>[4x]MAGTST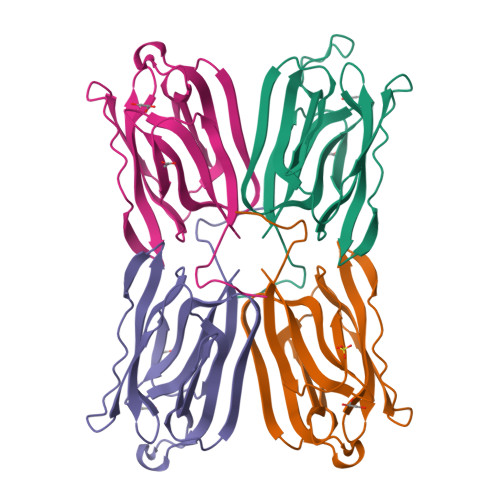NTQTTGTSQTIEVGLWGGPGGNAWDDGSYTGIREINLSHGDAIGAFSVIYDLNGQPFTGPTHPGNEPSFKTVKITLDFPNEFLVSVSGYTGVLARLATGKDVIRSLTFKTNKKTYGPYGKEEGTPFSLPIENGLIVGFKGRSGFVVDAIGFHLSL> MLQEQSELMSTVMNNTPTTVAALAAVAAASETNGKLGSEEQPEITIPKPRSSAQLEQLLYRYRAIQNHPKENKLEIKAIEDTFRNISRDQDIYETKLDTLRKSIDKGFQYDEDLLNKHLVALQLLEKDTDVPDYFLDLPDTKNDNTTAIEVDYSEKKPIKISADFNAKAKSLGLESKFSNATKTALGDPDTEIRISARISNRINELERLPANLGTYSLDDCLEFITKDDLSSRMDTFKIKALVELKSLKLLTKQKSIRQKLINNVASQAHHNIPYLRDSPFTAAAQRSVQIRSKVIVPQTVRLAEELERQQLLEKRKKERNLHLQKINSIIDFIKERQSEQWSRQERCFQFGRLGASLHNQMEKDEQKRIERTAKQRLAALKSNDEEAYLKLLDQTKDTRITQLLRQTNSFLDSLSEAVRAQQNEAKILHGEEVQPITDEEREKTDYYEVAHRIKEKIDKQPSILVGGTLKEYQLRGLEWMVSLYNNHLNGILADEMGLGKTIQSISLITYLYEVKKDIGPFLVIVPLSTITNWTLEFEKWAPSLNTIIYKGTPNQRHSLQHQIRVGNFDVLLTTYEYIIKDKSLLSKHDWAHMIIDEGHRMKNAQSK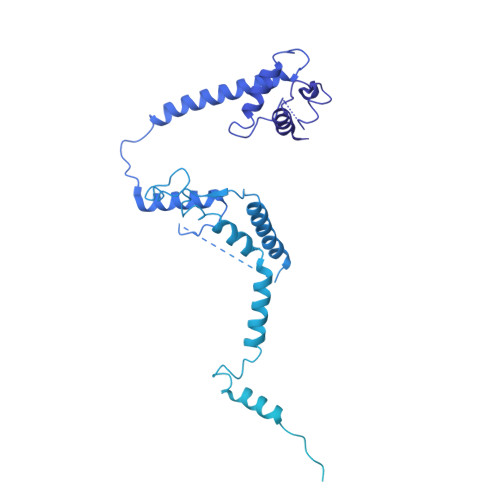LSFTISHYYRTRNRLILTGTPLQNNLPELWALLNFVLPKIFNSAKTFEDWFNTPFANTGTQEKLELTEEETLLIIRRLHKVLRPFLLRRLKKEVEKDLPDKVEKVIKCKLSGLQQQLYQQMLKHNALFVGAGTEGATKGGIKGLNNKIMQLRKICNHPFVFDEVEGVVNPSRGNSDLLFRVAGKFELLDRVLPKFKASGHRVLMFFQMTQVMDIMEDFLRMKDLKYMRLDGSTKTEERTEMLNAFNAPDSDYFCFLLSTRAGGLGLNLQTADTVIIFDTDWNPHQDLQAQDRAHRIGQKNEVRILRLITTDSVEEVILERAMQKLDIDGKVIQAGKFDNKSTAEEQEAFLRRLIESETNRDDDDKAELDDDELNDTLARSADEKILFDKIDKERMNQERADAKAQGLRVPPPRLIQLDELPKVFREDIEEHFKKEDSEPLGRIRQKKRVYYDDGLTEEQFLEAVEDDNMSLEDAIKKRREARERRRLRQNGTKENEIETLENTPEASETSLIENNSFTAAVDEETNADKETTASRSKRRSSRKKRTISIVTAEDKENTQEESTSQENGGAKVEEEVKSSSVEIINGSESKKKKPKLTVKIKLNKTTVLENNDGKRAEEKPESKSPAKKTAAKKTKTKSKSLGIFPTVEKLVEEMREQLDEVDSHPRTSIFEKLPSKRDYPDYFKVIEKPMAIDIILKNCKNGTYKTLEEVRQALQTMFENARFYNEEGSWVYVDADKLNEFTDEWFKEHSS> GSHMITLTTDFGLKGPYVGEMKVAMLRINPNAKIVDVTHSVTRHSILEGSFVMEQVVK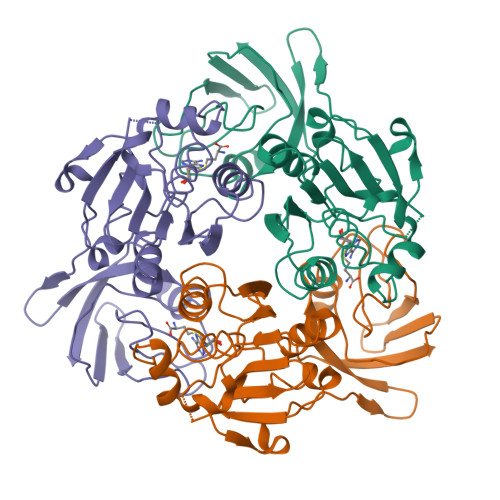YSPKGTVHVGVIDPGVGTERRAIVIEGDQYLVVPDNGLATLPLKHIKVKSVYEIIPDKIRKFTGWEISSTFHGRDIFGPAGALIEKGIHPEEFGREIPVDSIVKLNVEPRKEGDVWILKVIYIDDFGNVILNLENYEKPRTVELLDFNLRLPYLETYGLVEKGEMLALPGSHDYLEIAVNMGSAAERLNVKVGDELRVRLL> MQTPSIIQCGLLNSFARKMTDAISDNQIIATSRFFNIARDVADVVVSNTKLAQQYEQLSIDSLKEYLVSVAKFVAVDYSNTTSADVDDLIHKLRLFIEEECYQYNIDKEETCDGDVCVSDEYNEPAPKPKPKPKPKPAPKPKPAPKPKPAPKPAPKPAPKPAPKPAPKPAPKPAPKPAPEPAPEPAPEPAPKPAPEPAPEPAPIRPARRCDENPSNLETCCTNKALYGDFTDSSCDIVKKKTNWWLWGGIAILVIVLMIGGYFIYKRYFSAPKFENTGEFVNDMNFNNDVNFNNDVNFDNDMNYGNEGIDVSDLEILNLPVPSVSPVPSASIVPSVSPIPRGSPVPSASPIK;> MKTETLYQDPVWFQDLSVIFKRPSEIIPTRDQSDSERINAMVRLVLYCSFAVALIRQNYLYAILGLAIIAIISLAYALGAKKTKSNEAYGNIRPYSVKRSKKSCSKSSANNPFSNATVGALLDNEARPPACSYDDNDMASTMRKNFNKGLFRNLDDVYEVENSQRQFYTMPVTTAAPDLTAFGQFLYGSKGKTCKEDPSACTPAFATRDG;>MMNFILVLLIVAMIGTILVSESKYLFSKPVCKNCGVKAVTLPVDISAGKLAKVAEAVKKQTEEIKTLLKQKQSAPKAPELTNPIEHIKASTTVVSGANGLENVIDEDLPFSDFKGVPVAETTVEGMIKGIRPPTYADPRVMNPALAAAPVQFSDPTQFGTFGVTDDVSPAFSTEDKIPKTNAKISSDISVEGYENSYDANGARLVMDGKVVKSECQLPSYQIRNSKHHTQLPMRSLNEPPPMVEDLVDESLFEGLQGYPVDEKLDLLTPPGTATPSSEWAAINYGLTNN[2x];> MQIYSEYYEKIGPRKLRLLVKRRLLFASTWLYINNYILLSIIMKLQTKHMILLGFVAVVVVFIIFMLTRKKKEGFSIGNIFGKVKGAVTGTVGKVVNVVKPQGYKPEFVNRVNFGKFWACPEGTTDWGSEDKQCLVSQYGPMMWRNKGGNEWGWSCPAGSAPNNSDDWNQKCVQGYSMKKLIDGQWRCTDTEIDTGKDWSNSDWFTAQQQCDRGNNKVFTRRMYIDGKWQCPDGTWDTGFTWSDGENGGKQCKYYP;> MILVGIAVLILLAVFAILYYKQKEKFVVVGKFVEPIPSNPGQDFTLLPMDQTYTFADPVPDTATAFDVVLSRFTDKKAPADLLKGATFPEAAPYTDSEVENISKLALSRVKGPDAPVLSFISVEYAAKGVDNKKNTHYDIAFMVYDQVKNFSLKLVLVAVLDAKNKLWIKKFSSFNSFTPKDKGPKGVENIDETPLAEFIPDFVQFSRLYKDNANV;> MVETTQHFVSIESSNRPDPANTTPANYSIQLPQRYRNIWSAMLVNIALPAVSPPQKYVYLDIDKLNSIDSTSPSGGVNFALAKIPLSIAGTGNVFFADTMTSSFPNVPLQNPVATMDKLNIKLKDANGNVLTIPAGNEHSFMIQLTCGDYIPRGGGSTITQNGRVLGGTR;> MGNGPPMERAVSSDDILTYYNTFIFFIYFNFTNENIYIIYTIYMKVQNTIVYIVLLLIVVVIIWNFTRKEGWSDYNAPNDFMKIYYSNIVEDKKLAEKYPFFGTGPFTGLRCRKPNNVGCNTTWVSGQLVELTPKLKEQIECKFGIQYVKT;> MDSRLSAAYAIRAARISMIPGGVDGLVINYAEGGEPAWVQYPLKKQKPLPNNLCYTPTLEDIARKREAVIAKYTKQPLETGTTFTHVLNASHLNEQYTRVKKSALPDKEFPIIETEKYPEPPILWETTIGAPSRLFDRSDGVKYVR;>[12x]MDMHMIVKVVAILAVLFLVYKLWESMNKPNASPLKIQNPYEKYMNSAEGGEYDAEDDDIYYPETDAEDDDIYTGETDDMYDGEDDDIYVQEGDDIEDAEDEPYDDSADMEQDVPKVQQPMMPLLTPSSQLLPKPSPEAADFAQFAPKNLQAQNFLTATQWIGVNTQGSSLKNANYDLRADPIIPKADVGPWMMSSVDPNIYQKPLFG;> MCNTYYKRVKFNLFLYTNSIEMELLAVASIIGYGLFSSQQGRETRPDRNRYAEALGSGQGLDEDYDVKPTDMVRKYRKKAEKRWKKAQVPKESGIITPNMRPSEVMPYFTSGKSMNTNTDYKQRKMELFTGGVLDGHSVSGTYKHKVEAANMFGMTPQGRVTSDGTVGNAPGDTELLKARSVNSHQYNNVLPTEQLRVGPGLGVGPEVAATGGFHQFYRQLPLNINEYKLTQLPGRLVPGGTTTGGKGEIQQIASVNHNPDALVLNYDDRPPEATPNGAILASTQYGKQPRGYAGLRPYEKNYEGIAEADVSALQARYLDQTRGRPRTGDGDTEPIINPNGERDGTGSYVTENMCSMTLESQRGLVNRYITPPGVTGVVQQGGEMRPEFVPETTIREQYEDIYYTGPAGTTVTPTEPMNVVELQPESRHAKRAGQDRAYTPGAGRVNNFAPAAQGAYGLKDHPTYNALQHVVSEPIEQTFLPAAQGDDDRFGTKSNVNNPWGNPASLQIANNQLAANKFNRDVTNTVNLDYDAGQPMKQQNFQPKAWIPNNTDDMKMLPLWKRKQLQAQKNKQQRK;>MFSAFRDTASIGFSDTHQDEKTLRFLKKQISQFIKHLKEYYPNNELTKKLVMKYSDVQLLPYTKGATKDTYTSGLFDHTTGVIKIAPRDGLGNVRDEQSLNKSICHELAHGTRVKYPGESSHSDEWKDAWKTFLKIAADELGWKIEVPCSSVSFYGLTKDDCENCVWDQDPETCPKTAKLA[4x];>[3x]MAMKTQRKENVLFQNVKPREIPLVDNPFSTYPYKHVITETQPTQAKNQAIWGLVQMGLSGEAAAMYGDVVVQKTTRACRKSEGGFKDVNTELWGTSPYLGRGDGEVYNMPASNQLLRGFESSLRGSRVRTQIDDKSFIPYTWQMIDVPLAAAKTSFIAGLDTRQQLAYGNP;> METIGNFIQNMAFPTENPYKLSGDFGNSTLEPTVTAALRILHESPAPFNTEFFSRKNVDFIQKKLISETKRYTSFDIGPQNEDELIMMMAGIYVQDSTFDGNIKAGLRKLNTLVITECLKQILPGVRAYALYVRDASLPFSGGGEEAFKRPELATLKGSKVLSGFLPLDRNAS;>MAGGLSQLVAYGAQDVYLTGNPQITFFKTVYRRYTNFAIESIQQTINGSVGFGNKVSTQISRNGDLITDIVVEFVLTKGGNGGTTYYPAEELLQDVELEIGGQRIDKHYNDWFRTYDALFRMNDDRYNYRRMTDW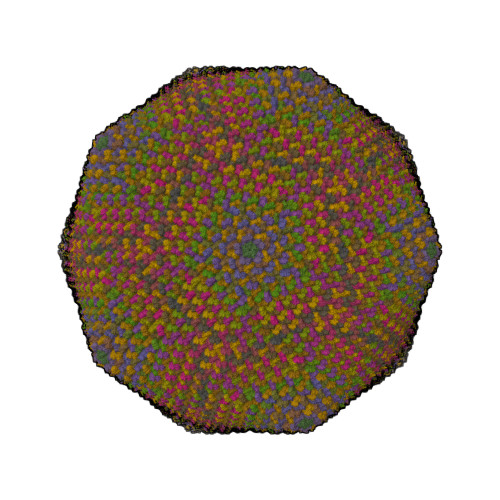VNNELVGAQKRFYVPLIFFFNQTPGLALPLIALQYHEVKLYFTLASQVQGVNYNGSSAIAGAAQPTMSVWVDYIFLDTQERTRFAQLPHEYLIEQLQFTGSETATPSATTQASQNIRLNFNHPTKYLAWNFNNPTNYGQYTALANIPGACSGAGTAAATVTTPDYGNTGTYNEQLAVLDSAKIQLNGQDRFATRKGSYFNKVQPYQSIGGVTPAGVYLYSFALKPAGRQPSGTCNFSRIDNATLSLTYKTCSIDATSPAAVLGNTETVTANTATLLTALNIYAKNYNVLRIMSGMGGLAYAN[84x];> MHKITPFLIAAVVAVIVLAVWLFKKDNKKETWFSRDLNYGKANSKIWNATVAKGLKGIANENAEIRKMYPYLGYGDFTGAICKGPNNQGCTYYANYTR> MHHHHHHAMAQLGEMVTVLSIDGGGIRGIIPATILEFLEGQLQEMDNNADARLADYFDV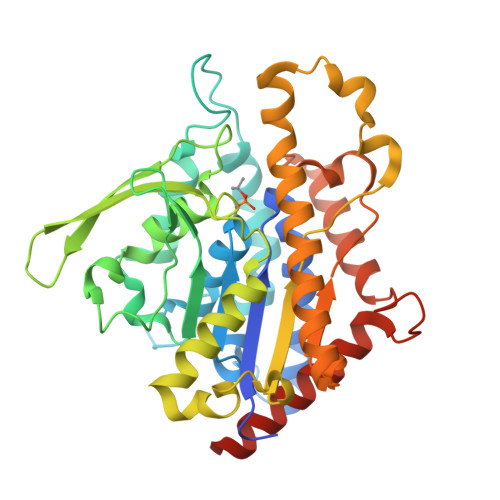IGGTSTGGLLTAMISTPNENNRPFAAAKEIVPFYFEHGPQIFNPSGQILGPKYDGKYLMQVLQEKLGETRVHQALTEVVISSFDIKTNKPVIFTKSNLANSPELDAKMYDISYSTAAAPTYFPPHYFVTNTSNGDEYEFNLVDGAVATVADPALLSISVATRLAQKDPAFASIRSLNYKKMLLLSLGTGTTSEFDKTYTAKEAATWTAVHWMLVIQKMTDAASSYMTDYYLSTAFQALDSKNNYLRVQENALTGTTTEMDDASEANMELLVQVGENLLKKPVSEDNPETYEEALKRFAKLLSDRKKLRANKASY> PK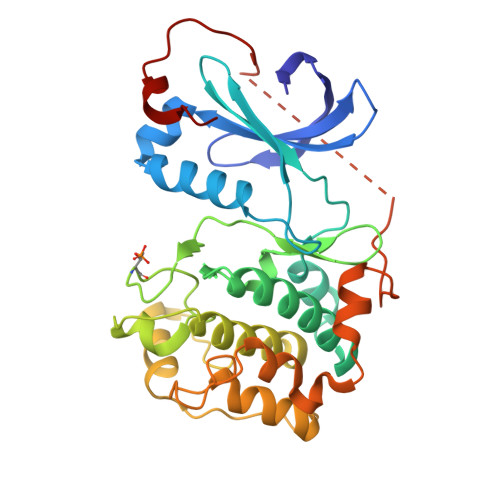YSLQDFQILRTLGTGSFGRVHLIRSRHNGRYYAMKVLKKEIVVRLKQVEHTNDERLMLSIVTHPFIIRMWGTFQDAQQIFMIMDYIEGGELFSLLRKSQRFPNPVAKFYAAEVCLALEYLHSKDIIYRDLKPENILLDKNGHIKITDFGFAKYVPDVTYTLCGTPDYIAPEVVSTKPYNKSIDWWSFGILIYEMLAGYTPFYDSNTMKTYEKILNAELRFPPFFNEDVKDLLSRLITRDLSQRLGNLQNGTEDVKNHPWFKEVVWEKLLSRNIETPYEPPIQQGQGDTSQFDKYPEEDINYGVQGEDPYADLFRDF We determined the full-length structures of two members (Fl8CE20_II and PpCE20_II) from the carbohydrate esterase family 20 (CE20) by X-ray crystallography that feature an ancillary domain, inserted into the catalytic SGNH-hydrolase domain. Detailed structural analysis identifies a so far undescribed catalytic triad architecture which lacks the typical aspartate for polarization of the histidine but instead reveals a precisely coordinated water molecule mediating contact between the His and Asp. This coordinated water in the Ser-His-(H2O-Asp/Asn) motif, as further confirmed by mutational studies and by determination of kinetic constants, is crucial for catalytic activity. We therefore term this active site architecture a water-mediated catalytic triad.

Fl8CE20_II was previously proven to solely act as a de-O-acetylase on acetylated xylans. The ancillary domain of Fl8CE20_II has a β-sandwich fold, composed by eight antiparallel β-strands, reminiscent from β-galactosidases of the GH2 family (PFAM PF02837 or PF13364). In both crystal structures of Fl8CE20_II and PpCE20_II, representing the only structures of CE20 enzymes featuring the inserted ancillary domain solved so far, the Asp (Fl8CE20_II: Asp513; PpCE20_II: Asp518) carboxylate has a distance to the catalytic His Nδ of 4.0 Å which is too far away for a direct interaction. Instead, the Asp side chain contributes to precisely coordinating a water molecule (Fl8CE20_II: 2.9 Å), which is in direct hydrogen bond distance to the catalytic His base (Fl8CE20_II: 2.9 Å). The tetrahedral coordination geometry of this water molecule is completed by interaction with a main chain carbonyl oxygen of Tyr334 in the ancillary domain and by another water molecule. Moreover, besides coordinating the water molecule, Asp513 in the SGNH hydrolase domain forms a direct salt bridge to Lys370 of the ancillary domain. Thus, Asp513 has a dual function, i.e., a catalytic role in coordinating and positioning the catalytic water molecule and a structural role in binding and orienting the ancillary domain with direct consequences on substrate binding. As expected, the mutation Asp513 to Ala in Fl8CE20_II (D513A) resulted in complete inactivation of the enzyme showing the importance of this residue for catalysis. In conclusion, we could clearly show that the active site Asp/Asn side chain of Fl8CE20_II is in fact, crucial for catalytic activity, while it is, in contrast to a conventional triad, not directly interacting with the His.

>[2x]MKKINLLLFIALQCVFSVSSAQIKLPKLVSDGMVLQRDTPVNLWGWSKPQEVISIVFAEKNYTTRADSEGNWKLKLDATPAGGPYTIALSASNTITLNDVVFGDVWLCSGQXNMELPMSRVSPLYEDEIASANNAEIRYFEVPKTYDFKEEKQDITFGKWEKVTPETIENFSAVAYFFAKNLNAELQVPIGLINSSLGGSPAEAWISEEGLKKFPEYYTEAERFKDNDLIDSIEQSDQTRRDTWYKTLNDTDQGIINNWKSADFDFSGWKIMNIPGYWAATEIGDKNGSVWFKKQVEIPKKWLNRPIKLLMGRIVDADSIFVNDTFIGNTTYQYPPRRYEIPAGILRDGKNTITVRVLNESGKGGFVEEKPYKLVMDEQEIDLRGKWHYKLGSEMPFLQGQTFIRWKPEGLYNAMIAPFTSMNLKGVIWYQGESNADTPAEYQELFTTLIEDWRSKWNAPEFPFLFVQLANFMATKEEPGDSNWARLRDAQRRTLAVPHTGMAVTIDIGEGNDIHPLNKKDVGDRLAQAAKHVAHGKNVVAGSPLYDSMEIEGDTIIIRFKNTGSGLMAKNGKPGYFAIAGEDQKFIWADAVIKDDKILVSSPAIKNPVAVRYGWADNPEGANIYNKEGFPASPFRTDNW> MVAAFSYTACTKLSLLHPSMVAQIRPRTTQKAFVVTNPEQDSTLEVQETETLKEEQSTEKMKKQPTPLRPVEKQLNVKSKGMGDFGGQWLSSVTRHVRIYAAYIDPETCEFDQSQMDKLTLILDPTEEFVWDDESCNKVYSYFQELVDHYEGAPLTEYTLRLIGSDVEHYIRKM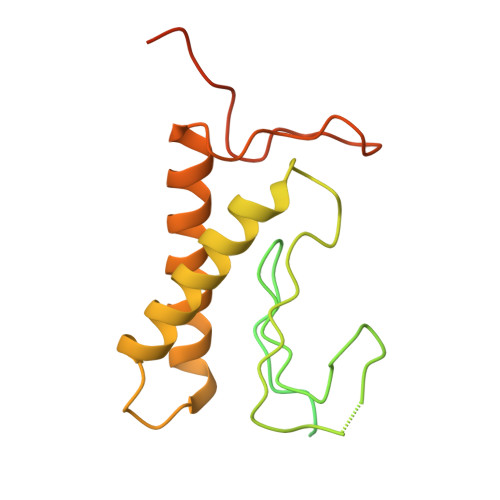LFDGEIQYNMDARVLNFSMGKPRVQFNTSNIEGGGDGQPQEDA>MGKTQLFPDSPLTDQDFSQLDQTVIDTARRQLIGRRFIELYGPLGRGIQSIFNDVFIENYEAKMDFQGSFDTDIETSKRVNYTIPLLYKDFVLYWRDLEQAKVLDIPIDFSAAANAARDVAILEDQMIFYGSKEFDIPGLMNVKGRSTHLIGNWYESGNAFQDVVEARNKLLEMKHNGPFALVLSPELYSLLHRVHKDTNVLEIEHVRELVTDGVFQTPVLKGKTGVLVNTGRNNLDLAVSEDFDTAYLGEEGMNHPFRVYETVVLRIKR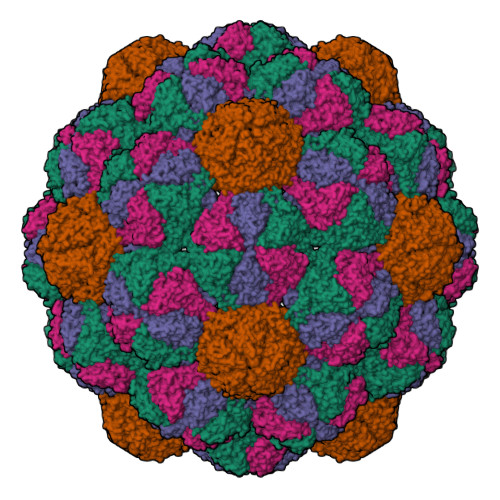PSAICTLEDGGE[4x]> MASMTGGQQMGMPAITCVWSDGRSDTWPNVNGHSRTRSVPSLKPLPHQDSKNLLYRQICGRLLAQHVFGGAGSTQPILNQLCKRLSTGNPNNTNASTVVTAPEKNVVSARHVRPNPKSSKDTLEKQPKYSSQIYLTDSFENYYLASLPTNYQLYQRDSNRENGNGKREFWLYGHPSGRPFRSVND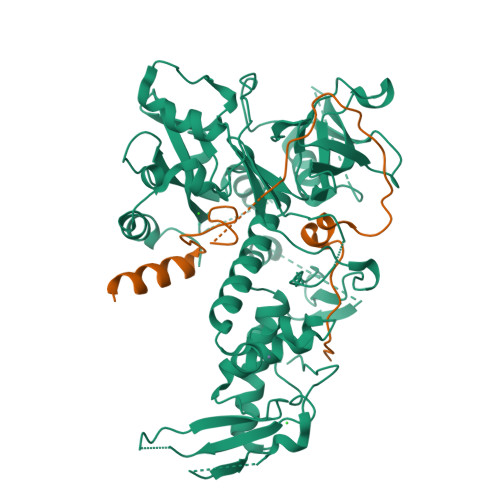FLHHLYWLISDLTRNESTCCCVLCSGNMTRVRKNLQKENERMFHECKDDTYTWPSSYRLGEVVWIDINNELIPAIIVARNLINYESNQMDAVKLISDTFVEPYQYHCKQLGNSRYYFDMAAADIEPWSRHPLDLQKQEHLVAHSICQTWNLFGIFQPLEGIDMEEPKFHDENYSIPLTVLPTFGGESNSLDDHFYGIFRGAEKLWINDLCVISTSSLPSVLQKTSFMYISDIYVNEDDIVCFQGSLWTQIDKNALDYNDSADNIDEHKDDLKELPRRLQMVSKLSNTYFRCLHDKSVEYVCPFADVLGRWYEPWFVKGDLNYTSEVKERTSSRLSAVGSENWVDDDFYEYLLSEIDMVSAVVM;> SSLLSRLTQSNQSKDKIIAALAKRNVYKSFAGLYDSKGKNDNTGYDFDSNYARVGRHGSFILPVSKSVPTPSLLIEGSIVQRKNIKIE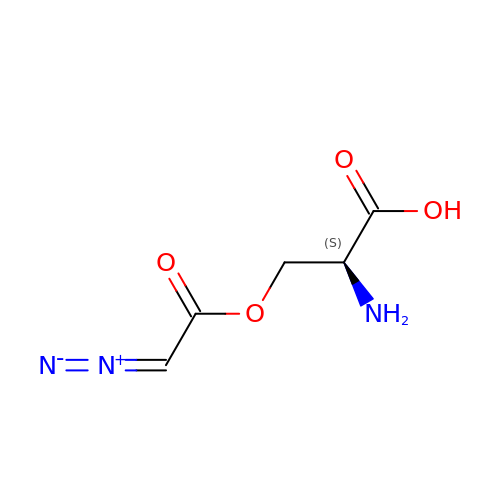O-DIAZOACETYL-L-SERINE | C5 H7 N3 O4 | MZZGOOYMKKIOOX-VKHMYHEASA-N>MTVAKAIFIKCGNLGTSMMMDMLLDE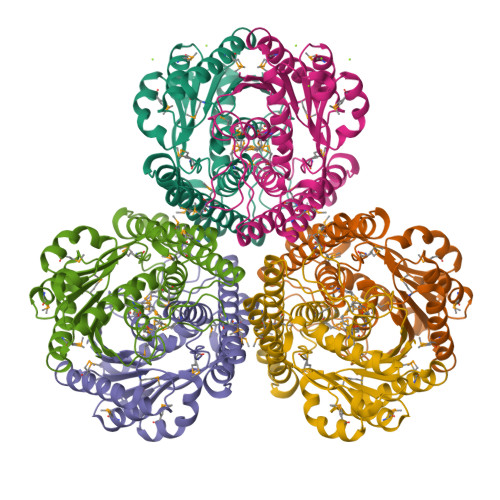RADREDVEFRVVGTSVKMDPECVEAAVEMALDIAEDFEPDFIVYGGPNPAAPGPSKAREMLADSEYPAVIIGDAPGLKVKDEMEEQGLGYILVKPDAMLGARREFLDPVEMAIYNADLMKVLAATGVFRVVQEAFDELIEKAKEDEISENDLPKLVIDRNTLLEREEFENPYAMVKAMAALEIAENVADVSVEGCFVEQDKERYVPIVASAHEMMRKAAELADEARELEKSNDAVLRTPHAPDGKVLSKRKFMEDPE[3x]> APNAEVIVVEGPREKVKGKITELVKELKERGKKVGVIGSESYNADEFFFLGSSVEEVAKNLF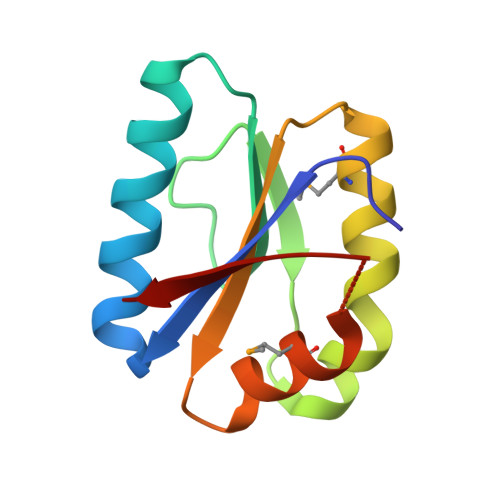KALRYMDKAGVDVVIAEGVEERGLGLAVMNRLRKASGYKIVKA Cyclic β-1,2-glucan (CβG) is a circular polysaccharide critical for host interactions of many bacteria, including major pathogens of humans (Brucella) and plants (Agrobacterium). The production of the main CβG chain occurs in the cytoplasm and is orchestrated by the cyclic glucan synthase (Cgs), a large, multi-domain membrane protein that contains several enzymatic sites. We determine the structure of this complex protein machinery and clarify key aspects of CβG synthesis, revealing a distinct mechanism that uses a tyrosine-linked oligosaccharide intermediate in cycles of polymerization and processing of the glucan chain.

In addition, catalytically inactive mutants of the GT (CgsiGT) and GP (CgsiGP) domains were generated by introducing substitutions of the predicted active site residues (D624A/D626A/D739A and D2393A/D2528A, respectively). The CgsiGP mutant displays reduced flexibility compared to CgsWT, resulting in improved cryo-EM maps obtained from smaller datasets: CgsiGP1 for the APO dataset, CgsiGP2 for the UDP-Glc dataset, and CgsiGP3 for a subset of the UDP-Glc dataset. Models CgsiGP1 and CgsiGP2 indicate that the presence of UDP-Glc affects the gating loop conformation. In the apo state, the loop can be found above the GT active site. Our cryo-EM maps contain a polysaccharide density attached to the residue Y694, which is a part of the IF1-homology loop. The density corresponds to a chain of minimum 8–9 glucose molecules that interacts with the tetratricopeptide (TPR) homology motif of the NTD.

> DHNDSIRASYMTIEELHDAGAALSRDGADSLPGFMEFDFFERHRENEKEILRVYRTTAVDAENGATITPAAEWLLDNHYVIEEAIQEVRRDFPRKFYRQLPTMTVGGVTIPRVMALGWLYVAHTHSTVSRENMTALVDGYQTSQTLQIGELWALPSIIRFVLIENLRRISIRVERSRRMRQKANEVVDEIIRLNDAEASAALLKQVDSLVDDPTFATQFLYRLRNGSQTSGFAVAWLEERLHAAGTDAENVMMSEHNRLASGNVTMGNIVKSLREIDDTEWSVWFEEVSHIDKVLREETDYEILDFGSRNTYRNTIELLARRSPRTEVEVARAAVEMARSDLPAGADENHRVNVGSVLVGQRRFELEKALGYRPLASQHIVRSMRKFNWLAIAAPVLLITAVAMLAVGWFLAKAGMPWYVVTAFLLMFALPASEGATGLFNTLVTFFVKPFRLVGYEFKNGIPEDARTLVAVPCMLTSRDSVDEMMRNIEVHYLANPHGEIYFSLVSDWRDAPYEQSDEDLEILDYAKRELAALNSRYAFDGKTRFYLLHRRRIYNSAEECWMGWERKRGKLHELNMLLRGDKDTTFLGGSNIVPADVKYVMTLDADTRLMRDAVTKLVGKMHHPINRPKIDPVSGRVVEGYGLLQPRVTPSLTTGKDASVFQRVFSINRGIDPYVFTVSDVYQDLTSEGTFTGKGLYDVDAFEAALKGRIEENSILSHDLLEGSFARCALVTDVELVEDFPTRYEVEVSRQHRWARGDWQLLPFIIDRARGVTAIGRWKMVDNLRRSLTPIAWFFASILGWYFMDPLGALIWQILLIFSLFVAPTLSLLSGLVPRSTDIVPQAHFFTIWSEIRATNAQVALRIVFIADAACMMTDAIVRSLYRLLVSHKLMLEWRTAASMQSSAQGSIVDYYRQMWHAPVVAMLGLLFAALPGDNAFLIGIPFTLLWVLSPAVAWYVSQSAETEDRLFVSEHVSFELRKIARRTWRYYEAFVTPQENHLPPDNFQETPEPIVASRTSPTNIGVYLLSVISARQFGWISFADTLERIENTIQTVEKMEKHRGHLYNWYHTDTLQTLGPRYVSAVDSGNLAGHLIAVSSACRDWAEAPSAHLQGNLDGIGDVAGILRETLKALPDNRKTLRPLHRRLEERIIGFSNALASVKREHEFASIRVINLAVLARDIQKLATNVDHEVKSAQSAEVTRWAQLLVESCEAHISDSAIDLTNMEPLRQRLASLRDRSRNLAFSMDFTFLYRKDRRLLSIGYRVESKELDEACYDLLASECRLTSLFAIAKGDLPTEHWYRLGRQVVPIGAQGALVSWSGSMFEYLMPPLVMQERQGGILNQTNNLIVKEQMNHGRRLGTPWGISEAAFNARDHNMNYQYTNFGVPTLGLKRGLGQNAVIAPYASILASQYDPDGALENLDKLRKLGALGQYGFHDAVDFTPTRVPDGKVCAVVYNYYAHHHGMSIAAVANVAFDGVLRELFHSDPVIEAAELLLQEKAPREVPVMSAKYEPETPGKEQADLLRAEVRSIADPAVRDREVVFLSNGHYSTMLTSTGAGYSKWNGQAISRWKADPTDDRWGTFIFLRDTTNGQWWSATAEPRVIEGEKTKTIFTDDKAEFHKTIGDLQSVVECIVATEHDAEGRRITLLNVGSEDRYIEVTSYMEPVIASEDDDNAHPLFSRMFVQTEIGRRGDVIRAWRNRRSQNEPGTVIAHLAADNAGPSRPTEFETDRAKFIGRGRSLREAAAFDAGATLSSSDGFTLDPILSLRRTVRVPAGKKVSVIFWTIAAPSREEVDKAIDRYRHPDAFAHELVHAWTRTQVQMRHVGVTSQQAAAFQHLGRYLTYPDMHLRADSETLKTGLASQRALWPLAISGDFPIFSLRINDDMDMDIAREALSAHEYLRSRGVIFDLVIVNERAASYAQDMQHALDHISETQRRINPADGGRPHVFSVRRDLMDEETWSALLAASRVVLHVRNGKIVDQINRAVSLFAANRGPDGSSDAAQARLPVPAFPVAEPVEDAGDLDFWNGFGGFAKNGQEYVVRLNGGQSTPHPWINVISNENFGFHISAEGAGFSWSRNSRDYQLTPWTNDPVINRPGEAFYVADVETGKLYTPCAALSRDPEAMFETRHGLGYSILTGVADTLEVELTQTVDREKPVKFSQVIVRNKGSKSRRLKVYAYVEWVLGNNGQKSAPFILSRHDAGSNAIFASNPYSIDYSARTSFLTLDSEASGFTTSRREFIGRFGSAQAPQGIVAGAALSGTTEVDGDPCAALMQEIHLKPGEERHMTFILGDADNAEEAEALVKDVRQADFLSVLEESKKFWTGFTGQLQVSTPDAGFNHMVNNWLPYQALACRILARTAFYQSSGAFGFRDQLQDTLAFLLYQPDLARTQILRAAGRQFPEGDVQHWWLPLTGAGVRTTISDDVVWLAYAINQYVSATGDAAILDESIPFLKGPALMPGQHDAFFQPETSERSATLYEHAALALDLAIHRTGENGLPLILGGDWNDGMNRVGVGGKGTSVWLGWFLAGALRDFIEIAEKRGDTDRVGKWASHREKLRHVLETAGWDGSYYRRGYFDDGTPLGSASSEECQIDSLGQSWSVLSGEGEEGRSRQAMDAVMEHLVDEKTGIIRLFTPPFSRASHDPGYIKGYPPGVRENGGQYTHAATWVVLALAKQGRAQEAWNCFKLLNPVNHALDAASSETYRVEPYVVTADVYGEGAYAGRGGWSWYTGSAGWLYRAAVEGILGITRTDGKLHVSPSLPEDWSGFSIRITLDGKARDIAVSRKAGTADVSVSVDG>[2x]LKQINHQGEEEELIALNLSEARLVIKEALVERRRAFKRSQKKHKKKHLKHENANDETTAVEDEDDDLDEDDVNADDDDFMHSETREKELESIDVLLEQTTGGNNKDLKNTMQYLTNFSRFRDQETVGAVIQLLKS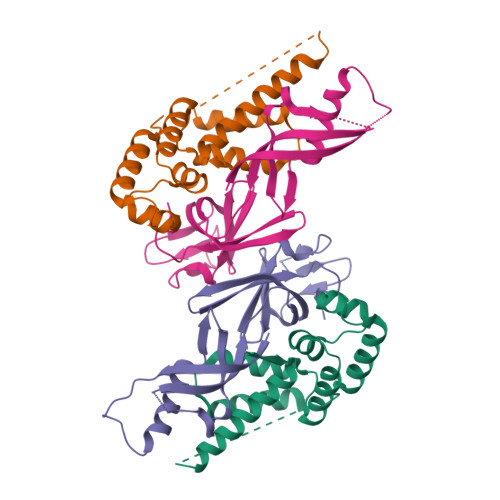TGLHPFEVAQLGSLACDTADEAKTLIPSLNNKISDDELERILKELSNLETLY;>MFFIKDLSLNITLHPSFFGPRMKQYLKTKLLEEVEGSCTGKFGYILCVLDYDNIDIQRGRILPTDGSAEFNVKYRAVVFKPFKGEVVDGTVVSCSQHGFEVQVGPMKVFVTKHLMPQDLTFNAGSNPPSYQSSEDVITIKSRIRVKIEGCISQVSSIHAIGSIKEDYLGAI[2x]N-[(2S)-3-amino-1-(hydroxyamino)-3-methyl-1-oxobutan-2-yl]-4-[4-(4-aminophenyl)buta-1,3-diyn-1-yl]benzamide | C22 H22 N4 O3 | 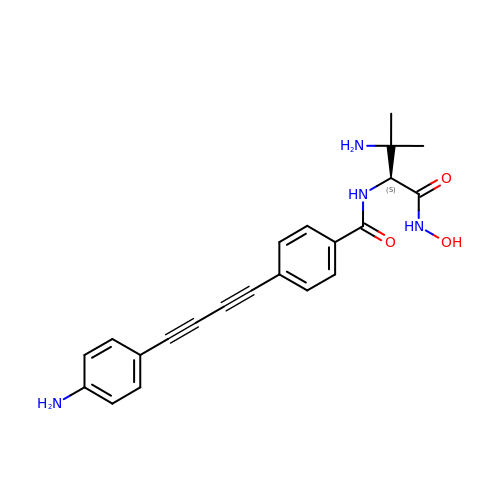VVHQDGBAFRDCKP-LJQANCHMSA-N>[2x]SMVRRTKEEAQETRAQIIEAAERAFYKRGVARTTLADIAELAGVTRGAIYWHFNNKAELVQALLDSLHETHDHLARASESEDEVDPLGCMRKLLLQVFNE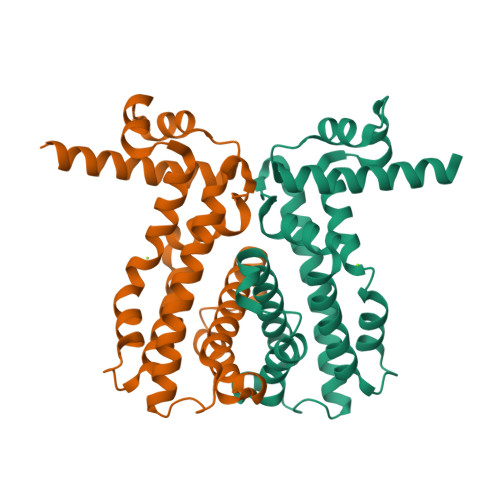LVLDARTRRINEILHHKCEFTDDMCEIRQQRQSAVLDIHKGWTLALANAVRRGQLPGELDAERAAVALYAYVDGLIRRWLLLPDSVDLLGDVEKWVDTGLDMLRLSPALRK Bacterial cellulosic polymers constitute a prevalent class of biofilm matrix exopolysaccharides that are synthesized by several types of bacterial cellulose secretion (Bcs) systems, which include conserved cyclic diguanylate (c-di-GMP)-dependent cellulose synthase modules together with diverse accessory subunits. In E. coli, the biogenesis of phosphoethanolamine (pEtN)-modified cellulose relies on the BcsRQABEFG macrocomplex, encompassing inner-membrane and cytosolic subunits, and an outer membrane porin, BcsC. Here we present cryo-EM structures of the E. coli Bcs macrocomplex positioning all seven BcsRQABEFG partners and multiple c-di-GMP-binding sites.

We demonstrate that BcsA’s N-terminal domain adopts an amphipathic fold to recruit three copies of the pEtN-transferase BcsG, stabilized opposite of the previously reported hexameric BcsB crown. Indeed, using local refinement to resolve the more dynamically associated pEtN-transferase, we show here that BcsANTD adopts an amphipathic fold and recruits three copies of the BcsG pEtN-transferase whose transmembrane N-terminal domains are tightly packed between BcsATMD and the sixth BcsB protomer of the crown, whereas the C-terminal catalytic BcsG modules remain unresolved in the structures. The BcsA N-terminus folds into a W-shaped series of amphipathic α–helices whose connecting loops coordinate the BcsG protomers via conserved amino acid motifs in an otherwise weakly conserved primary structure. The first and second BcsB copies engage in contacts with the BcsA synthase, where the C-terminal TA of BcsB1 fits in a groove formed by BcsA TMα1–3 and is further encased by BcsANTD to complete the membrane export module, while BcsB2-TA engages in limited hydrophobic contacts with the loop connecting BcsA TMα3 and TMα4 at the periplasmic side of the inner membrane. Interestingly, in BcsG the amphipathic helical loops point outwards relative to the crown’s lumen, where BcsB’s stacked carbohydrate-binding domains are proposed to form the polysaccharide extrusion path. This suggests major conformational gymnastics of the catalytic C-terminal domains for pEtN extraction and transfer onto the nascent cellulosic polymer, and could potentially explain the lack of resolved BcsGCTD-corresponding regions in the averaged electron density maps. The evolution of enterobacterial BcsANTD for the recruitment of multiple BcsG copies per synthase could thus provide efficient substrate mining for extensive polymer modification during processive synthase activity, where individual BcsG protomers are likely to act independently of each other. The membrane sampling and significant conformational changes, which would be required for pEtN-transfer onto a nascent polymer processively extruded through the periplasmic BcsB crown, are possibly enabled by the 48 amino-acid long interdomain linker that could at least theoretically extend more than 10–15 nm in the periplasmic space.

> MSILTRWLLIPPVNARLIGRYRDYRRHGASAFSATLGCFWMILAWIFIPLEHPRWQRIRAEHKNLYPHINASRPRPLDPVRYLIQTCWLLIGASRKETPKPRRRAFSGLQNIRGRYHQWMNELPERVSHKTQHLDEKKELGHLSAGARRLILGIIVTFSLILALICVTQPFNPLAQFIFLMLLWGVALIVRRMPGRFSALMLIVLSLTVSCRYIWWRYTSTLNWDDPVSLVCGLILLFAETYAWIVLVLGYFQVVWPLNRQPVPLPKDMSLWPSVDIFVPTYNEDLNVVKNTIYASLGIDWPKDKLNIWILDDGGREEFRQFAQNVGVKYIARTTHEHAKAGNINNALKYAKGEFVSIFDCDHVPTRSFLQMTMGWFLKEKQLAMMQTPHHFFSPDPFERNLGRFRKTPNEGTLFYGLVQDGNDMWDATFFCGSCAVIRRKPLDEIGGIAVETVTEDAHTSLRLHRRGYTSAYMRIPQAAGLATESLSAHIGQRIRWARGMVQIFRLDNPLTGKGLKFAQRLCYVNAMFHFLSGIPRLIFLTAPLAFLLLHAYIIYAPALMIALFVLPHMIHASLTNSKIQGKYRHSFWSEIYETVLAWYIAPPTLVALINPHKGKFNVTAKGGLVEEEYVDWVISRPYIFLVLLNLVGVAVGIWRYFYGPPTEMLTVVVSMVWVFYNLIVLGGAVAVSVESKQVRRSHRVEMTMPAAIAREDGHLFSCTVQDFSDGGLGIKINGQAQILEGQKVNLLLKRGQQEYVFPTQVARVMGNEVGLKLMPLTTQQHIDFVQCTFARADTWALWQDSYPEDKPLESLLDILKLGFRGYRHLAEFAPSSVKGIFRVLTSLVSWVVSFIPRRPERSETAQPSDQALAQQGSARSSGRTGLEFEEFYPYDVPDYAADYKDDDDKRS;>MTQFTQNTAMPSSLWQYWRGLSGWNFYFLVKFGLLWAGYLNFHPLLNLVFAAFLLMPLPRYSLHRLRHWIALPIGFALFWHDTWLPGPESIMSQGSQVAGFSTDYLIDLVTRFINWQMIGAIFVLLVAWLFLSQWIRITVFVVAILLWLNVLTLAGPSFSLWPAGQPTTTVTTTGGNAAATVAATGGAPVVGDMPAQTAPPTTANLNAWLNNFYNAEAKRKSTFPSSLPADAQPFELLVINICSLSWSDIEAAGLMSHPLWSHFDIEFKNFNSATSYSGPAAIRLLRASCGQTSHTNLYQPANNDCYLFDNLSKLGFTQHLMMGHNGQFGGFLKEVRENGGMQSELMDQTNLPVILLGFDGSPVYDDTAVLNRWLDVTEKDKNSRSATFYNTLPLHDGNHYPGVSKTADYKARAQKFFDELDAFFTELEKSGRKVMVVVVPEHGGALKGDRMQVSGLRDIPSPSITDVPVGVKFFGMKAPHQGAPIVIEQPSSFLAISDLVVRVLDGKIFTEDNVDWKKLTSGLHKQHRSPRTQMQ[3x];> TPATQPLINAEPAVAAQTEQNPQVGQVMPGVQGADAPVVAQNGPSRDVKLTFAQIAPPPGSMVLRGINPNGSIEFGMRSDEVVTKAMLNLEYTPSPSLLPVQSQLKVYLNDELMGVLPVTKEQLGKKTLAQMPINPLFITDFNRVRLEFVGHYQDVCENPASTTLWLDVGRSSGLDLTYQTLNVKNDLSHFPVPFFDPRDNRTNTLPMVFAGAPDVGLQQASAIVASWFGSRSGWRGQNFPVLYNQLPDRNAIVFATNDKRPDFLRDHPAVKAPVIEMINHPQNPYVKLLVVFGRDDKDLLQAAKGIAQGNILFRGESVVVNEVKPLLPRKPYDAPNWVRTDRPVTFGELKTYEEQLQSSGLEPAAINVSLNLPPDLYLMRSTGIDMDINYRYTMPPVKDSSRMDISLNNQFLQSFNLSSKQEANRLLLRIPVLQGLLDGKTDVSIPALKLGATNQLRFDFEYMNPMPGGSVDNCITFQPVQNHVVIGDDSTIDFSKYYHFIPMPDLRAFANAGFPFSRMADLSQTITVMPKAPNEAQMETLLNTVGFIGAQTGFPAINLTVTDDGSTIQGKDADIMIIGGIPDKLKDDKQIDLLVQATESWVKTPMRQTPFPGIVPDESDRAAETRSTLTSSGAMAAVIGFQSPYNDQRSVIALLADSPRGYEMLNDAVNDSGKRATMFGSVAVIRESGINSLRVGDVYYVGHLPWFERLWYALANHPILLAVLAAISVILLAWVLWRLLRIISRRRLNPDNE> GRAPDSVDYRK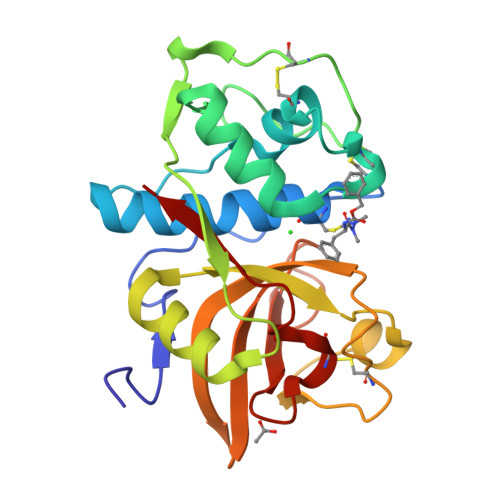KGYVTPVKNQGQCGSCWAFSSVGALEGQLKKKTGKLLNLSPQNLVDCVSENDGCGGGYMTNAFQYVQKNRGIDSEDAYPYVGQEESCMYNPTGKAAKCRGYREIPEGNEKALKRAVARVGPVSVAIDASLTSFQFYSKGVYYDESCNSDNLNHAVLAVGYGIQKGNKHWIIKNSWGENWGNKGYILMARNKNNACGIANLASFPKM> SMQFSKMHGLGNDFMVVDAVTQNVFFSPELIRRLADAHLGVGFDQLLVVEPPYDPELDFHYRIFNADGSEVAQCGNGARCFARFVRLKGLTNKRDIRVSTANGRMVLTVTDDDLVRVNMGEPNFEPSAVPFRANKAEKTYIMRAAEQTILCGVVSMGNPHCVIQVDDVDTAAVETLGPVLESHERFPERANIGFMQV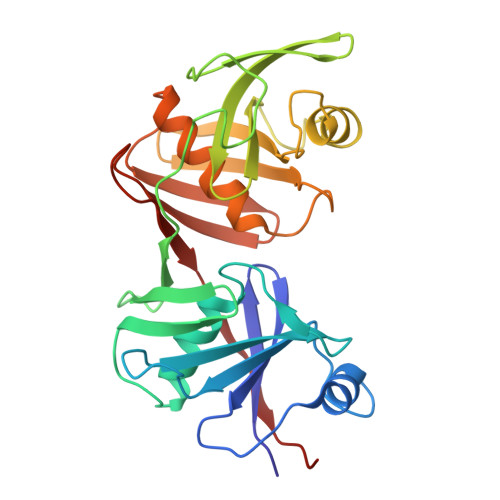VKREHIRLRVYERGAGETQACGSGACAAVAVGIQQGLLAEEVRVELPGGRLDIAWKGPGHPLYMTGPAVHVADGFIHL> HMLEDPMNKALKAL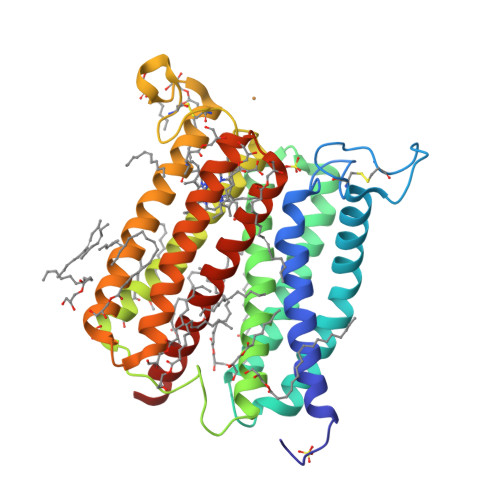GVLTTFVMLIVLIGGALVTKTGSGQGCGRQWPLCHGRFFPELNPASIIEWSHRFASGISIILVLSLAFWSWRKITPIFRETTFLAIMSIIFLFLQALLGALAVVFGSNALIMALHFGISLISFASVLILTLLIFEADKSVRTLVKPLQIGKKMQFHMIGILIYSYIVVYTGAYVRHTESSLACPNVPLCSPLNNGLPTQFHEWVQMGHRAAALLLFVWIIVAAVHAITSYKDQKQIFWGWISCLIFITLQALSGIMIVYSELALGFALAHSFFIACLFGVLCYFLLLIARFRYES> TSFAEYWN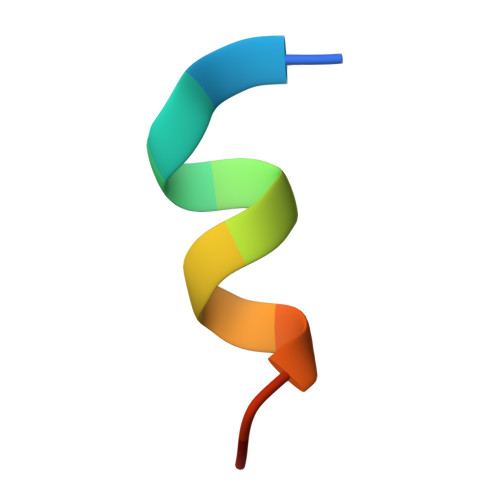LLSP> QDM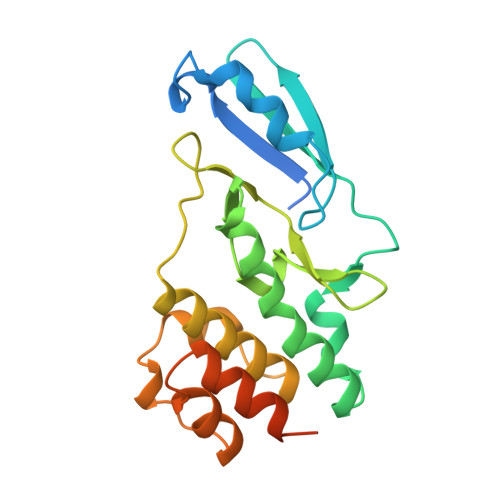LTPLDAEEAAKTKLRLDMREIPKSSIKPEHFHLMYLLEQHSPYFIDAELTELRDSFQIHYDINDNHTPFDNIKSFTKNEKLRYLLNIKNLEEVNRTRYTFVLAPDELFFTRDGLPIAKTRGLQNVVDPLPVSEAEFLTRYKALVICAFNEKQSFDALVEGNLELHKGTPFETKVIEAATLDLLTAFLDEQYQKQEQDYSQNYAYVRKVGHTV> MSCAGEALAPGPAEQQCPVEAGGGRLGSPAHEACNEDNTEKDKRPATSGHTRCGLMRDQSIWPNPSAGELVRTQPERLPQLQTSAQEPGKEETGKIKNGGHTRMSNGNGIPHGAKHVSVENHKISAPVSQKMHRKIQSSLSVNNDISKKSKVNAVFSPKAASSPEDCCVHCILACLFCEFLTLCNIVLGQASCGIC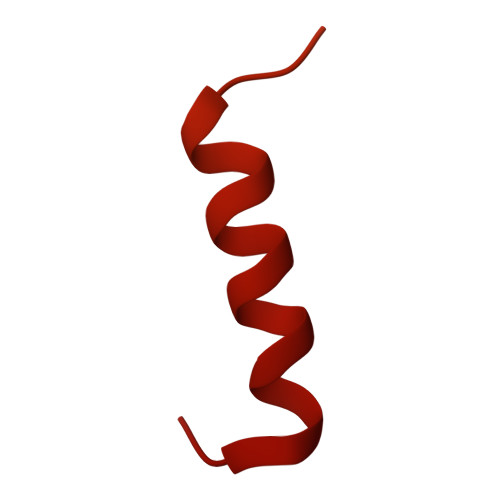TSEACCCCCGDEMGDDCSCPCDMDCGIMDACCESSDCLEICMECCGICFPS>MNTPEHMTAVVQRYVAALNAGDLDGIVALFADDATVENPVGSEPRSGTAAIREFYANSLKLPLAVELTQEVRAVANEAAFAFIVSFEYQGRKTV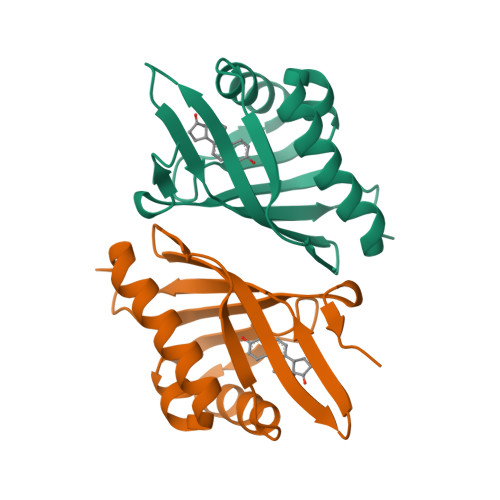VAPIDHFRFNGAGKVVSMRALFGEKNIHAGA[6x]>MDFVKELKSSQDYMNNELTYGAHNYDPIPVVLKRGKGVFVYDIEDRRYYDFLSAYSSVNQGHCHPDILNAMINQAKKLTICSRAFFSDSLGVCERYLTNLFGYDKVLMMNTGAEASETAYKLCRKWGYEVKKIPENSAKIIVCNNNFSGRTLGCVSASTDKKCKNNFGPFVPNFLKVPYDDLEALEKELQDPNVCAFIVEPVQGEAGVIVPSDSYFPGVASLCKKYNVLFVADEVQTGLGRTGKLLCTHHYGVKPDVILLGKALSGGHYPISAILANDDVMLVLKPGEHGSTYGGNPLAAAICVEALKVLI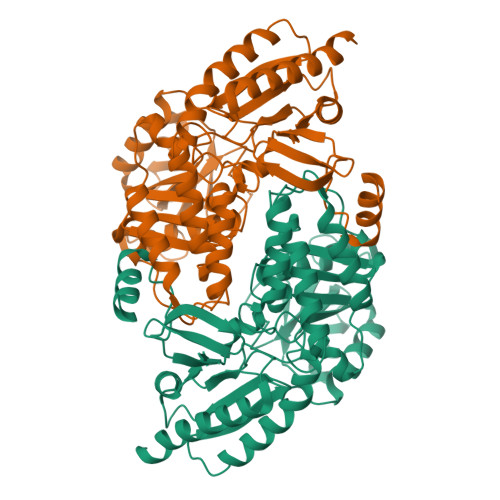NEKLCENADKLGAPFLQNLKEQLKDSKVVREVRGKGLLCAIEFKNDLVNVWDICLKFKENGLITRSVHDKTVRLTPPLCITKEQLDECTEIIVKTVKFFDDNLLQHHHHHH[4x]> NLIPTVIEQTNRGERAYDIYSRLLKDRIIMLGSAIDDNVANSIVSQLLF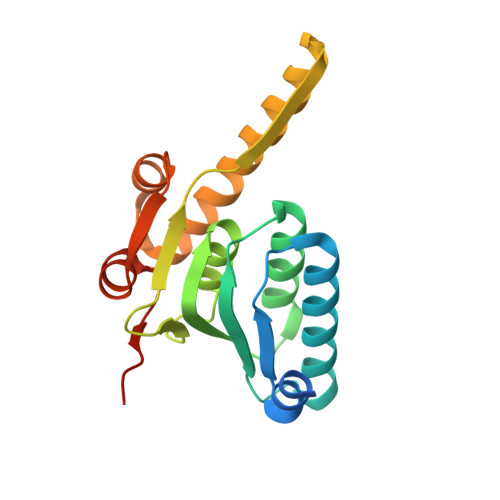LAAEDPEKEISLYINSPGGSITAGMAIYDTMQFIKPKVSTICIGMAASMGAFLLAAGEKGKRYALPNSEVMIHQPLGGAQGQATEIEIAAKRILLLRDKLNKVLAERTGQPLEVIERDTDRDNFKSAEEALEYGLIDKILTHTEDKKHHH>[4x]MHHHHHHSSGRENLYFQGYNEADVAALVRSLDRAEDHHIFAVDVLETYPYLAESYTKVCPRRCDLATAAQKALEGAYSYDLRLEGLKADIALMASNCVAYNGPTSAYAE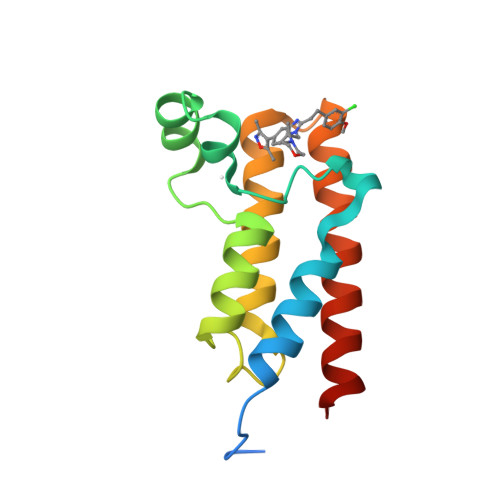TAAKFERYALEQIDAFVLEHNGGC>[4x]LTQELGTAFFQQQQLPAAMADTFLEHLCLLDIDSEPVAARSTSIIATIGPASRSVERLKEMIKAGMNIARLNFSHGSHEYHAESIANVREAVESFAGSPLSYRPVAIALDTKGPEIRTGILQGGPESEVELVKGSQVLVTVDPAFRTRGNANTVWVDYPNIVRVVPVGGRIYIDDGLISLVVQKIGPEGLVTQVENGGVLGSRKGVNLPGAQVDLPGLSEQDVRDLRFGVEHGVDIVFASFVRKASDVAAVRAALGPEGHGIKIISKIENHEGVKRFDEILEVSDGIMVARGDLGIEIPAEKVFLAQKMMIGRCNLAGKPVVCATQMLESMITKPRPTRAETSDVANAVLDGADCIML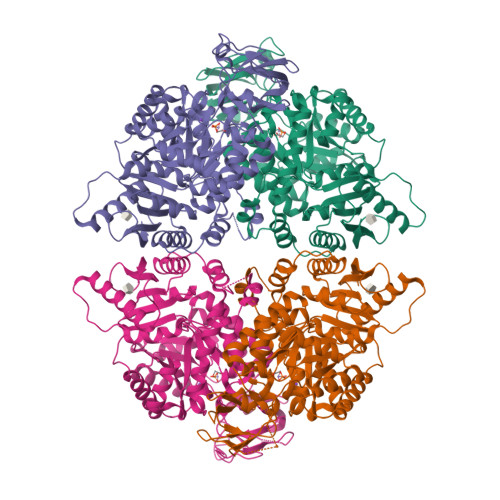SGETAKGNFPVEAVKMQHAIAREAEAAVYHRQLFEELRRAAPLSRDPTEVTAIGAVEAAFKCCAAAIIVLTTTGHSAQLLSRYRPRAAVIAVTRSAQAARQVHLCRGVFPLLYREPPEAIWADDVDRRVQFGIESGKLRGFLRVGDLVIVVTGWRPGSGYTNIMRVLSIS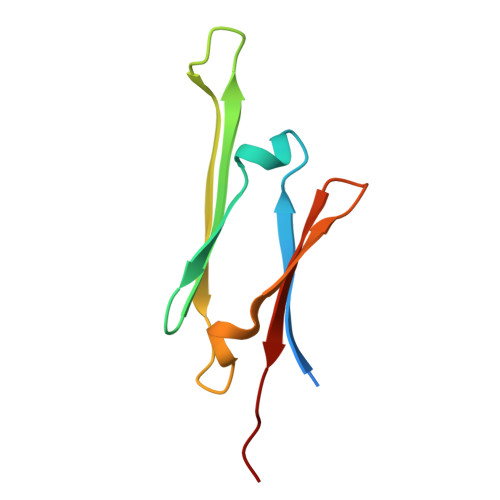> GSGNIKTLGDAYEFAVDVRDFSPEDIIVTTSNNHIEVRAEKLAADGTVMNTFAHKSQLPEDVDPTSVTSALREDGSLTIRARRHPHT>PMILGYWNVRGLTHPIRLLLEYTDSSYEEKRYAMGDAPDYDRSQWLNEKFKLGLDFPNLPYLIDGSRKITQSNAIMRYLARKHHLCGETEEERIRADIVENQVMDNRMQLIMLCFNPDFEKQKPEFLKTIPEKMKLYSEFLGKRPWFAGDKVTYVDFLAYDILDQYHIFEPKCLDAFPNLKDFLARFEGLKKISAYMKSSRYLSTPIFSKLAQWSNK[2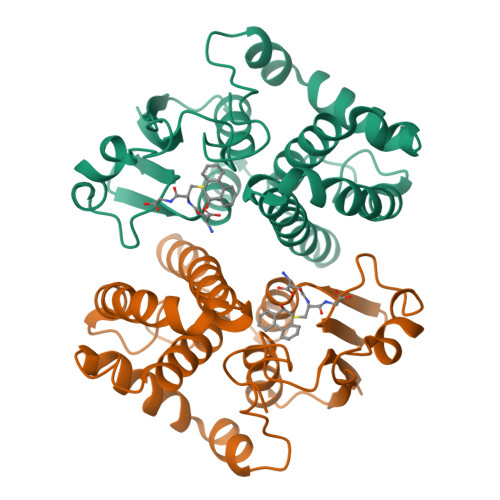x]>MFKLKLLSISTIFILAGCVSLAPEYQRPPAPVPQQFSLSKNSLTPAVNSYQDTGWRNFFVDPQVSRLIGEALNNNRDLRMAALKVEEARAQFNVTDADRYPQLNASSGITYNGGLKGDKPTTQEYDAGLELSYELDFFGKLKNMSEADRQN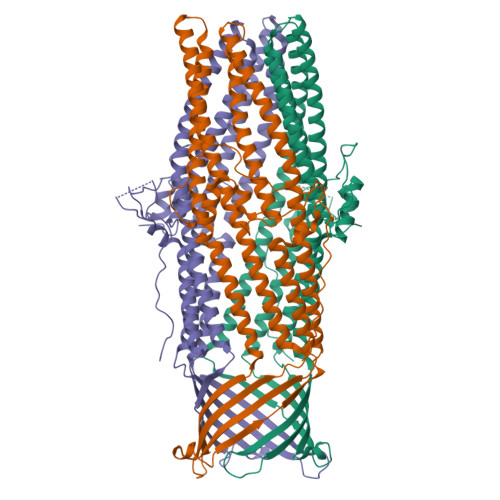YFASEEARRAVHILLVSNVSQSYFSQQLAYEQLRIARETLKNYEQSYAFVEQQLVTGSTNVLALEQARGQIESTRAEIAKREGDLAQANNALQLVLGTYRAVPSEKGIKGGEIAPVKLPPNLSSQILLQRPDIMEAEYQLKAADANIGAARAAFFPSITLTSGLSSSSTELSSLFTSGSGMWNFIPKIEIPIFNAGRNKANLKLAEIRQQQSVVNYEQKIQSAFKDVSDTLALRDSLSQQLESQQRYLDSLQITLQRARGLYASGAVSYIEVLDAERSLFATQQTILDLTYSRQVNEINLFTALGGGWVEK[5x];> MFKLKLLSISTIFILAGCVSLAPEYQRPPAPVPQQFSLSKNSLTPAVNSYQDTGWRNFFVDPQVSRLIGEALNNNRDLRMAALKVEEARAQFNVTDADRYPQLNASSGITYNGGLKGDKPTTQEYDAGLELSYELDFFGKLKNMSEADRQNYFASEEARRAVHILLVSNVSQSYFSQQLAYEQLRIARETLKNYEQSYAFVEQQLVTGSTNVLALEQARGQIESTRAEIAKREGDLAQANNALQLVLGTYRAVPSEKGIKGGEIAPVKLPPNLSSQILLQRPDIMEAEYQLKAADANIGAARAAFFPSITLTSGLSSSSTELSSLFTSGSGMWNFIPKIEIPIFNAGRNKANLKLAEIRQQQSVVNYEQKIQSAFKDVSDTLALRDSLSQQLESQQRYLDSLQITLQRARGLYASGAVSYIEVLDAERSLFATQQTILDLTYSRQVNEINLFTALGGGWVEKH>[12x]SMLTELIASNRRSAAIHAFVDTGLSTHFKDGIYVDISELSRKSGVNYARFSRLCDFLVEMGVLVSNDNKFRLSDECHVFANPESFESFMIKLEICSHYSNAWLMYGKS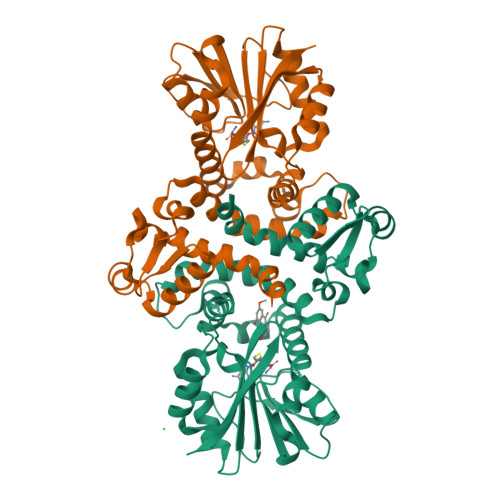LFEDDGKSAFEMAHGRPFFEYLDGNKFLKSNFDALMTRVSNLIVEKLLGIYDFNQHNRILDVGGGEGELLVRISEKVKGKHYAVLDRYSELPVSDNIDFINGNFLNSIPSGYDLYILKNVLHNWSDSDSILILENFRKAMDKNSSLLLINMVKEPEFSRSFDILMDVLFLGKERSFTEFEYLANQAGLVVQETKVIDQSYSPYSFIKLQIK>ANPYERGPDPTESSIEAVRGPFAVAQTTVSRLQADGFGGGTI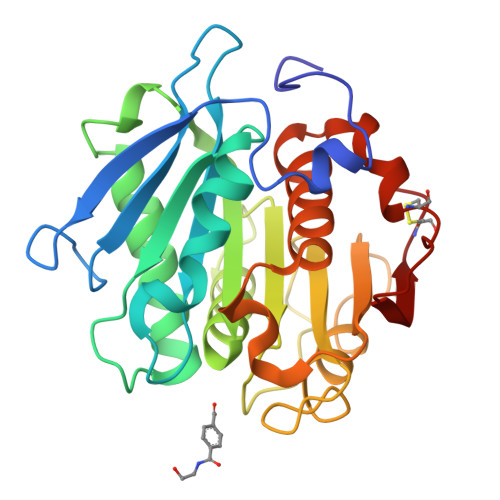YYPTDTSQGTFGAVAISPGFTAGQESIAWLGPRIASQGFVVITIDTITRLDQPDSRGRQLQAALDHLRTNSVVRNRIDPNRMAVMGHSMGGGGALSAAANNTSLEAAIPLQGWHTRKNWSSVRTPTLVVGAQLDTIAPVSSHSEAFYNSLPSDLDKAYMELRGASHLVSNTPDTTTAKYSIAWLKRFVDDDLRYEQFLCPAPDDFAISEYRSTCPF[2x]>[2x]MDEIKIEKLKKLDKKALNELIDVYMSGYEGLEEYGGEGRDYARNYIKWCWKKASDGFFVAKVGDKIVGFIVCDKDWF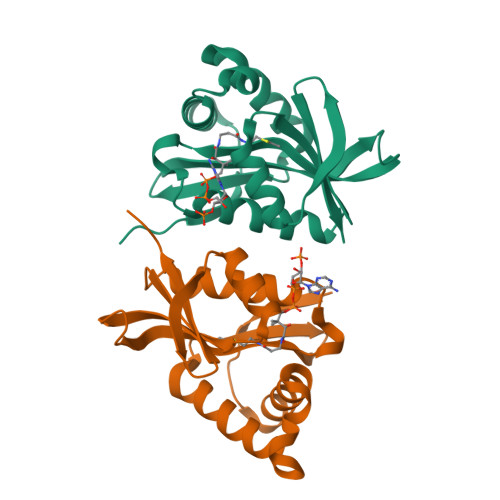SKYEGRIVGAIHEFVVDKKFQGKGIGRKLLITCLDFLGKYNDTIELWVGEKNYGAMNLYEKFGFKKVGKSGIWVRMIKRQNL> ALLVTAGIV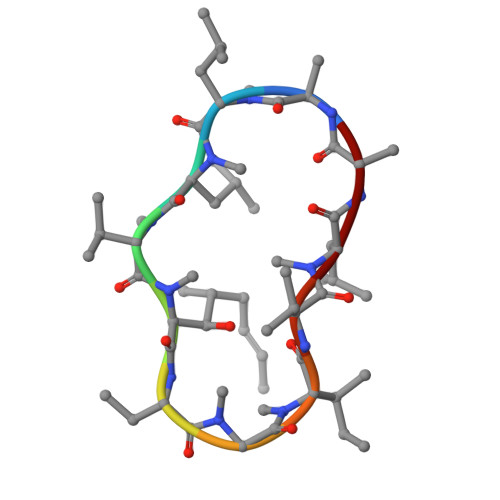LA> SDSSRRQYQEKYKQVEQYMSFHKLPPDTRQRIHDYYEHRYQGKMFDEESILGELSEPLREEIINFNCRKLVASMPLFANADPNFVTSMLTKLRFEVFQPGDYIIREGTIGKKMYFIQHGVVSVLTKGNKETKLADGSYFGEICLLTRGRRTASVRADTYCRLYSLSVDNFNEVLEEYPMMRRAFETVALDRLDRIGKKNSIL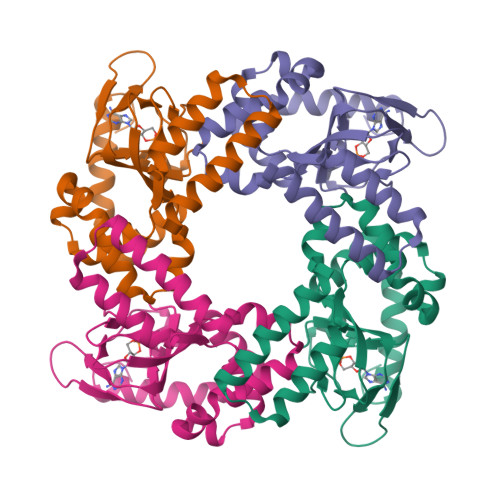LHKVQHDLNSGVFNYQEN1-(3,4-dimethoxyphenyl)-3-[3-(1H-imidazol-1-yl)propyl]thiourea 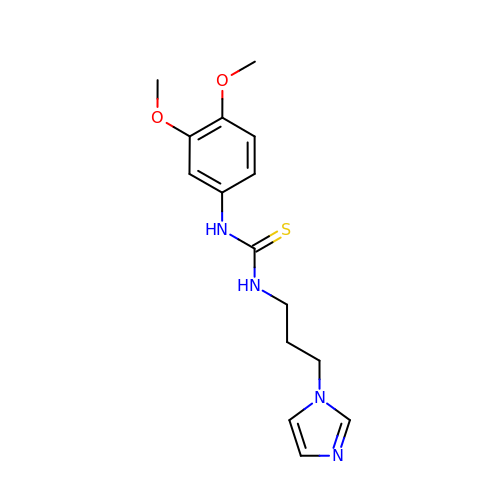| C15 H20 N4 O2 S | FZQXMGLQANXZRP-UHFFFAOYSA-N>[2x]SMNPIEDDLIFRVGTKGRNKGEFTNLQGVAASTNGKILIADSNNQCVQIFSNDGQFKSRFGIRGRSPGQLQRPTGVAVHPSGDIIIADYDNKWVSIFSS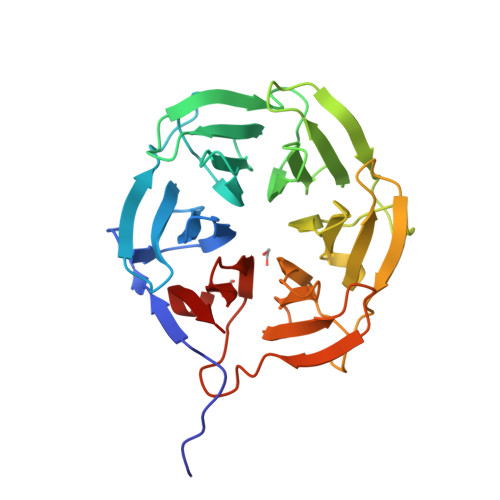DGKFKTKIGSGKLMGPKGVSVDRNGHIIVVDNKACCVFIFQPNGKIVTRFGSRGNGDRQFAGPHFAAVNSNNEIIITDFHNHSVKVFNQEGEFMLKFGSNGEGNGQFNAPTGVAVDSNGNIIVADWGNSRIQVFDGSGSFLSYINTSADPLYGPQGLALTSDGHVVVADSGNHCFKVY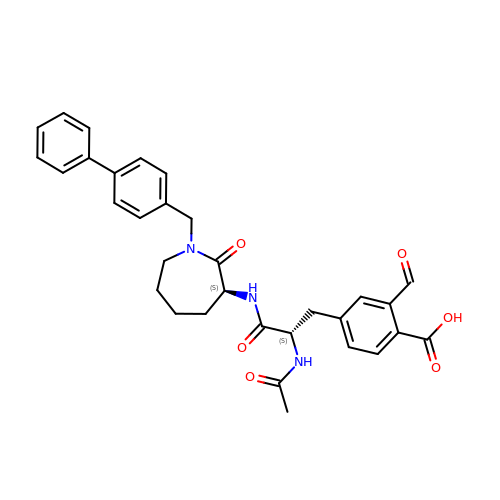4-[2-ACETYLAMINO-2-(1-BIPHENYL-4-YLMETHYL-2-OXO-AZEPAN-3-YLCARBAMOYL)-ETHYL]-2-FORMYL-BENZOIC ACID | C32 H33 N3 O6 | WKTQBTSOHBKBRW-VMPREFPWSA-N methyl (~{Z})-3-(4-ethynylphenyl)-2-methyl-prop-2-enoate 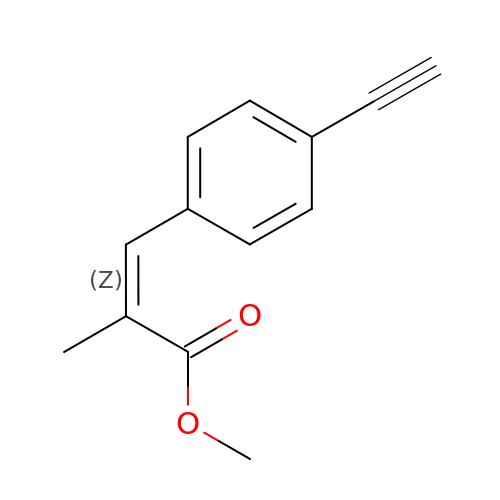| C13 H12 O2 | QXZSLVGPGBSCGY-KTKRTIGZSA-N> GSHMEIAATLQEIAKTLAEIAITLAEIAKTLKPESEEAKKAEEEAEKAAKEVEEAIKYAKEHPNSLEAVAKTLQAIAKTLATIAKTLAYIAKTLKPESEEAEKAEEEAKKAAERTEKAIKYAQAHPNSLEAVAKTLLAIAWTLAVIAWTLAYIAKTLDPESEEAEKAKKAAEEAKKKVEEAEKIAQKDPESLEAVAKTLAAIAATLAVI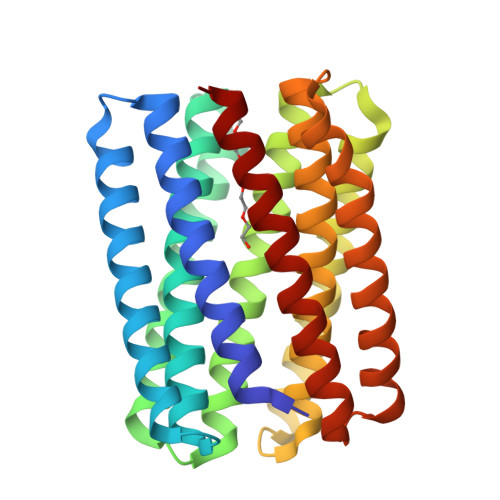AKTLAYIAKTLDPKSEEAKKAKEKAEAAAKKAAEAIEKAEKDPESLEAIAETLKAIADTLKVIAETLKTIAKTLK> MSKNRSSLQSGPLNSELLEEQKQEIYEAFSLFDMNNDGFLDYHELKVAMKALG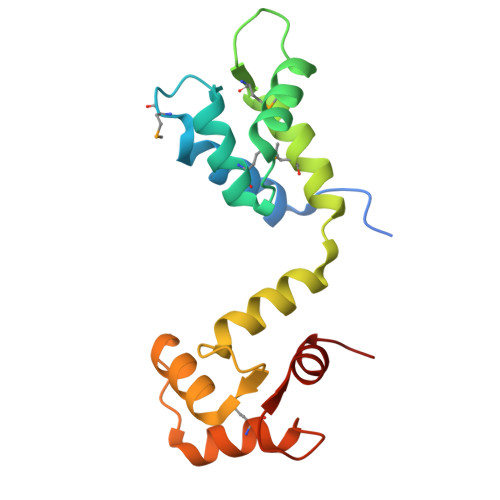FELPKREILDLIDEYDSEGRHLMKYDDFYIVMGEKILKRDPLDEIKRAFQLFDDDHTGKISIKNLRRVAKELGETLTDEELRAMIEEFDLDGDGEINENEFIAICTDS> MNLVLMGLPGAGKGTQAEKIVEKYGIPHISTGDMFRAAIKEGTELGLKAKSFMDKGELVPDEVTIGIVRERLSKDDCKKGFLLDGFPRTVAQAEALDNILSELGKKLDYVINIEVPKEELMER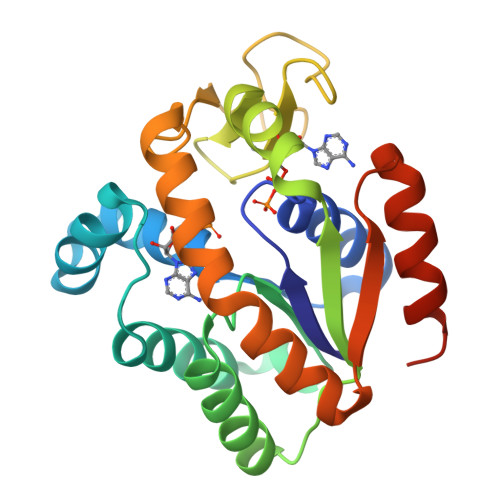LTGRRICKTCGATYHLIFNPPKVEGICDKDGGELYQRADDNPETVANRLDVNMKQTQPLLDFYEEKGVLRNIDGQQDINKVFADIKALLGGLKQENLYFQ>[2x]GHMETIHVGDRCLCRPGDRLGSVRFVGRVASLKPGYWVGVEFDEPVGKGDGTVKGTRVFQCQPNYGGFLRPDQVEVGDFPPEVF

Five tubulin-binding cofactors (TBCs) are implicated in late-stage tubulin folding and heterodimer assembly 1,5–10. TBC-B and TBC-E are implicated in binding α-tubulin, whereas TBC-A and TBC-D interact with β-tubulin. TBC-B comprises an N-terminal ubiquitin-like (Ubl) domain and a C-terminal cytoskeleton-associated protein with glycine-rich segment (CAP-Gly) domain.

Crystals of the CAP-Gly domain of TbTBC-B were obtained from a construct producing the 81 C-terminal amino acids. The crystals are orthorhombic with space group P212121, with two polypeptides, labelled A and B, in the asymmetric unit. The TbTBC-B CAP-Gly domain is a small globular structure with a similar fold to other CAP-Gly domains, and is an important module for the recognition and binding of the C-terminal tail of α-tubulin 17–18. The fold is dominated by five β-strands, β5–β9, forming a consecutive twisted antiparallel sheet with β9 returning to lie in an antiparallel fashion at the other side of β5. The side of strand β8 forms the floor of a solvent-exposed, primarily basic groove, which is flanked by the two extended loops, linking β6 and β7, and β7 and β8. The TbTBC-B CAP-Gly domain has a different sequence in this tubulin-binding motif at residues 195–199, GKGDG. Glycine rather than asparagine occupies the third position, and this nonconservative change precludes the formation of a side chain hydrogen bond with the terminal residue of an EE[Y/F] peptide. However, and fortuitously, in our structure the C-terminus of chain A forms intermolecular contacts with the basic groove of a symmetry-related chain B. The C-terminus of TbTBC-B has the sequence EVF, which is similar to the α-tubulin tail EE[Y/F] motif, and so these intermolecular interactions can be taken to mimic the association with a relevant binding partner. The peptide-binding groove on chain A is occupied by two formate molecules, derived from the crystallization mixture, which bind in similar fashion to the negatively charged moieties of the C-terminal peptide just discussed (data not shown).RIPK2 is an essential adaptor for NOD signalling and its kinase domain is a drug target for NOD-related diseases, such as inflammatory bowel disease. RIPK2 is an adaptor protein, which comprises a kinase and a caspase activation and recruitment domain (CARD) connected by a disordered intermediate loop. Among the IAPs, the X-chromosome-linked inhibitor of apoptosis, XIAP (also known as inhibitor of apoptosis protein 3 [IAP3] and baculoviral IAP repeat-containing protein 4 [BIRC4]) is thought to be the most critical ubiquitin ligase in the NOD2-RIPK2 signalling pathway. XIAP binds to the kinase domain of RIPK2 through its BIR2 domain.

Here, we present the structure of RIPK2 kinase bound to the BIR2 domain of XIAP determined by single-particle cryo-electron microscopy (SPA cryo-EM) at a nominal resolution of 3.15 Å. The final model of the complex corresponds to a mass of 84 kD, with a 2:1 stoichiometry, in agreement with both native MS and translational diffusion measurements by NMR. The structure shows that XIAP BIR2 binds at the RIPK2 dimer interface, interacting with the C-lobe of one kinase molecule (Kinase_A) and the N-lobe of the other one (Kinase_B). XIAP BIR2 uses loop 176–178 to mainly interact with Kinase_A and loop 209–214 to interact with Kinase_B. The XIAP BIR2 loop 176–178, which includes Y176 and H178, makes electrostatic interaction with the R36/R41 patch. The XIAP BIR2 loop 209–214 makes electrostatic interactions with the C-lobe of Kinase_B, which comprises residues belonging to the αH-helix (E279, S282, and K285) and to the regulatory region (K209 and I208). In particular, the two RIPK2 patches suggested to be part of the interaction, the R36/R41 basic patch and the regulatory region comprising K209, which are 40 Å apart in the monomer, are in fact close to each other in the dimer because of the antiparallel kinase arrangement. No interaction is observed between the XIAP BIR2 domain and the kinase activation loop, which indicates that XIAP binding requires RIPK2 to be in dimeric and αC-helix IN conformation, but not necessarily phosphorylated on the activation loop. Moreover, considering the RIPK2–XIAP BIR2 structure together with our biochemical and previously published observations, we confirm that K209 is critical for RIPK2 ubiquitination most likely because it contributes to the RIPK2–XIAP BIR2 interaction interface.

>MNGEAICSALPTIPYHKLADLRYLSRGASGTVSSARHADWRVQVAVKHLHIHTPLLDSERKDVLREAEILHKARFSYILPILGICNEPEFLGIVTEYMPNGSLNELLHRKTEYPDVAWPLRFRILHEIALGVNYLHNMTPPLLHHDLKTQNILLDNEFHVKIADFGLSKWRMMSLSQSRSSKSAPEGGTIIYMPPENYEPGQKSRASIKHDIYSYAVITWEVLSRKQPFEDVTNPLQIMYSVSQGHRPVINEESLPYDIPHRARMISLIESGWAQNPDERPSFLKCLIELEPVLRTFEEITFLEAVIQLKKTKLQSV[2x];> YPRNPAMYSEEARLKSFQNWPDYAHLTPRELASAGLYYTGIGDQVQCFCCGGKLKNWEPCDRAWSEHRRHFPNCFFVLGRNLNIRSE> IGMAPGGYVAPKAVWLPAVKAKGLEISGTFTHRQGHIYMEMNFTNKALQHMTDFAIQFNKNSFGVIPSTPLAIHTPLMPNQSIDVSLPLNTLGPVMKMEPLNNLQVAVKNNIDVFYFSCLIPLNVLFV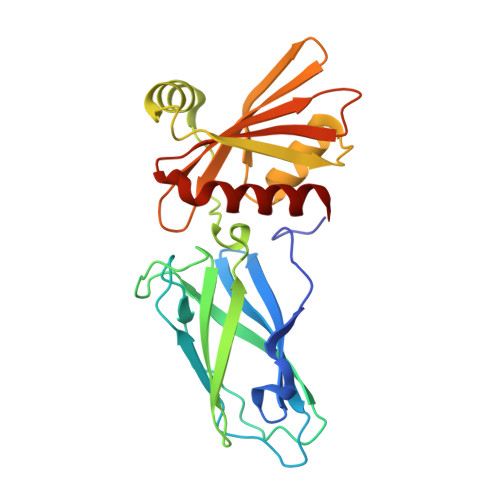EDGKMERQVFLATWKDIPNENELQFQIKECHLNADTVSSKLQNNNVYTIAKRNVEGQDMLYQSLKLTNGIWILAELRIQPGNPNYTLSLKCRAPEVSQYIYQVYDSILKN(7~{R})-2-[[3,5-bis(fluoranyl)-4-oxidanyl-phenyl]amino]-5,7-dimethyl-8-prop-2-ynyl-7~{H}-pteridin-6-one 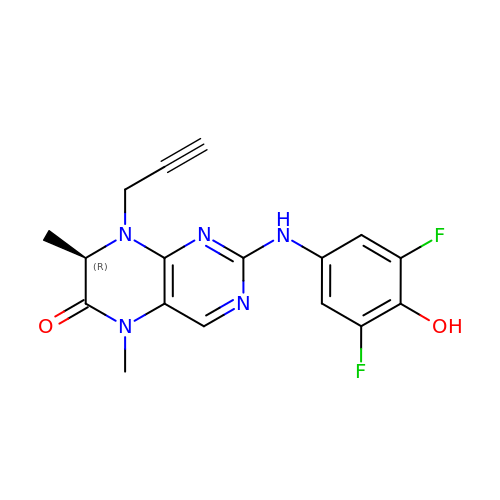| C17 H15 F2 N5 O2 | DYKLQWQETZOVEI-SECBINFHSA-N> MPAPAASGAAAVLSKDIARSFRWMQAFAAVKGKPTAGSCAAGTAVVNPEDPTKVTLKGRYTNFSLQHIWEKYDYLQTHL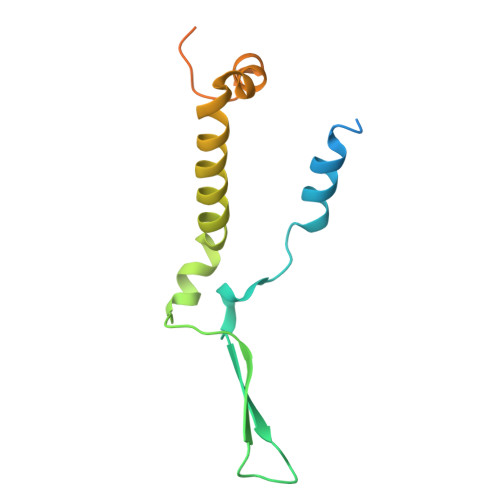LLRECMLSQVAKNPRLLDPEINAGLTPTVFMRVPPETQDPETQAKAAPQKGQAN> ADKELKFLVVDKFSTMRRIVRNLLKELGFNNVEEAEDGVDALNKLQAGGYGFVISDWNMPNMDGLE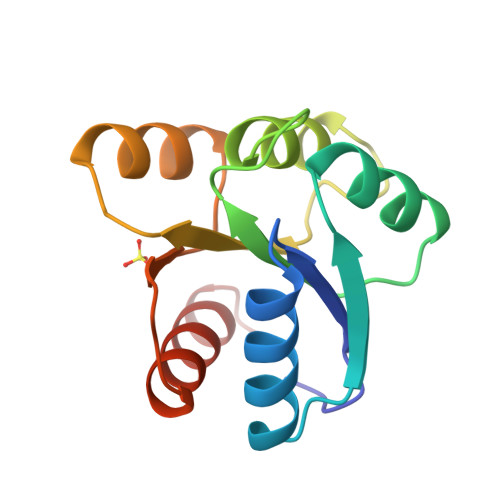LLKTIRADGAMSALPVLMVTAEAKKENIIAAAQAGASGYVVKPFTAATLEEKLNKIFEKLGM>ETGASAKELACQEITVPLCKGIGYEYTYMPNQFNHDTQDEAGLEVHQFWPLVEIQCSPDLKFFLCSMYTPICLEDYKKPLPPCRSVCERAKAGCAPLMRQYGFAWPDRMRCDRLPEQGNPDT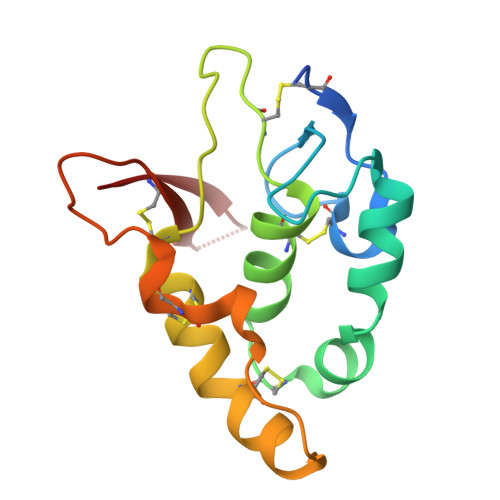LCMDYERGTLEVLFQG[4x]> GSLRQEDFPPRIVEHPSDLIVSKGEPATLNCKAEGRPTPTIEWYKGGERVETDKDDPRSHRMLLPSGSLFFLRIVHGRKSRPDEGVYVCVARNYLGEAVSHDASLEVAAAAHHHHHH;> GSLHCPAACTCSNNIVDCRGKGLTEIPTNLPETITEIRLEQNTIKVIPPGAFSPYKKLRRIDLSNNQISELAPDAFQGLRSLNSLVLYGNKITELPKSLFEGLFSLQLLLLNANKINCLRVDAFQDL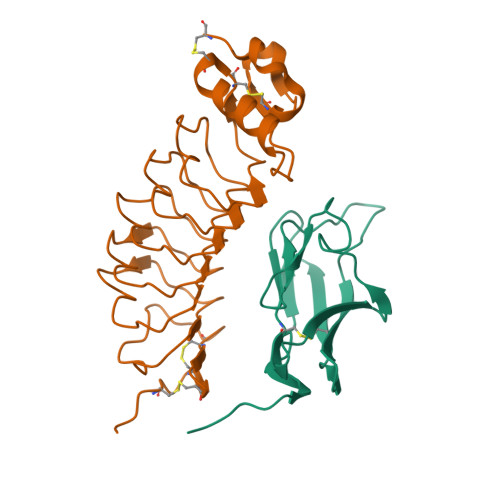HNLNLLSLYDNKLQTIAKGTFSPLRAIQTMHLAQNPFICDCHLKWLADYLHTNPIETSGARCTSPRRLANKRIGQIKSKKFRCSAAAHHHHHH> VVPPAGTPWGTAYDKAKAALAKLNLQDKVGIVSGVGWNGGPCVGNTSPASKISYPSLCLQDGPLGVRYSTGSTAFTPGVQAASTWDVNLIRERGQFIGEEVKASGIHVILGPVAGPLGKTPQGGRNWEGFGVDPYLTGIAMGQTINGIQSVGVQATAKHYILNEQELNRETISSNPDDRTLHELYTWPFADAVQANVASVMCSYNKVNTTWACEDQYTLQTVLKDQLGFPGYVMTDWNAQHTTVQSANSGLDMSMPGTDFNGNNRLWGPALTNAVNSNQVPTSRVDDMVTRILAAWYLTGQDQAGYPSFNISRNVQGNHKTNVRAIARDGIVLLKNDANILPLKKPASIAVVGSAAIIGNHARNSPSCNDKGCDDGALGMGWGSGAVNYPYFVAPYDAINTRASSQGTQVTLSNTDNTSSGASAARGKDVAIVFITADSGEGYITVEGNAGDRNNLDPWHNGNALVQAVAGANSNVIVVVHSVGAIILEQILALPQVKAVVWAGLPSQESGNALVDVLWGDVSPSGKLVYTIAKSPNDY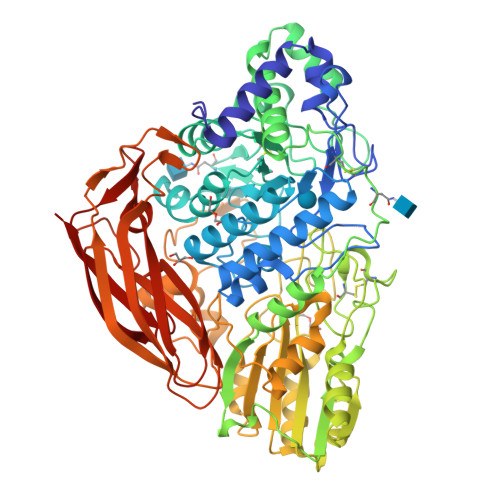NTRIVSGGSDSFSEGLFIDYKHFDDANITPRYEFGYGLSYTKFNYSRLSVLSTAKSGPATGAVVPGGPSDLFQNVATVTVDIANSGQVTGAEVAQLYITYPSSAPRTPPKQLRGFAKLNLTPGQSGTATFNIRRRDLSYWDTASQKWVVPSGSFGISVGASSRDIRLTSTLSVA>[4x]MASGCSTVDTVKDFNKDNFFTGSWYITHYKLGDSTLEVGDKNCTKFLHQKTADGKIKEVFSNYNPNAKTYSYDISFAKVSDFDGNNGKYTAKNVIVEKDGRKIDERTLQVSYIDTDYSKYS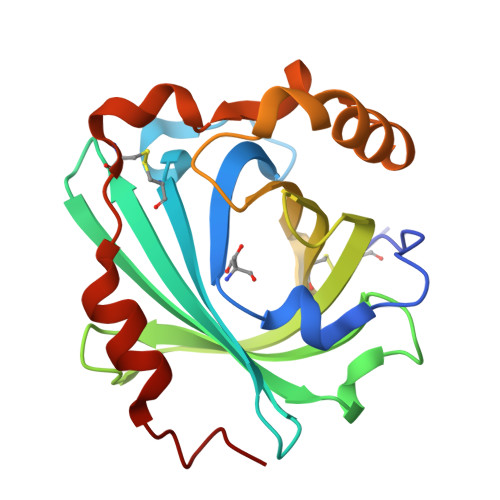VVHVCDPAAPDYYLYAVQSRTENVKEDVKSKVEAALGKVGLKLSGLFDATTLGNKCQYDDETLQKLLKQSFPNYEK In Neisseria gonorrhoeae, the best-characterized and most clinically important multidrug efflux system is the multiple transferrable resistance (MtrCDE) tripartite efflux pump, a member of the widely distributed resistance-nodulation-cell division (RND) superfamily in Gram-negative bacteria. N. gonorrhoeae MtrD contains multidrug binding sites and a proton relay network that generates the proton motive force (PMF) essential for drug expulsion from the bacterial cell. This multidrug efflux pump couples with the MtrC periplasmic membrane fusion protein and the MtrE outer membrane channel to actively extrude antimicrobials and mediate drug resistance. Based on the cryo-EM structures of MtrDCR103-CASP, MtrDCR103-Col, and MtrDCR103-LL, we observed that MtrDCR103 employs different binding modes to anchor linear and cyclic peptides.

To study MtrDCR103-Col interactions, we incubated 2 μM the MtrDCR103-nanodisc sample with 20 μM Col for 2 h to form the MtrDCR103-Col complex. We obtained a cryo-EM map of this complex at a 3.08-Å resolution. Similar to MtrDCR103-CASP, the structure of MtrDCR103-Col reveals an asymmetric trimer, with the three MtrDCR103 protomers exhibiting the access, binding, and extrusion conformational states. In the binding protomer of MtrDCR103, the cryo-EM map depicts an additional large density corresponding to the bound Col peptide. This bound Col molecule is found deep inside the distal drug binding site of the pump. The Col binding site overlaps that of CASP; however, it appears that MtrDCR103 utilizes a slightly different subset of residues to attach this peptide. Again, the nature of this protein-peptide interaction is mostly hydrophobic. Within 4.5 Å of this bound peptide, there are 26 residues, H46, S87, T128, S130, A132, S134, F136, I139, M141, Q172, R174, F176, S275, T277, A288, M290, P324, Y325, F568, I605, V607, F610, F612, S615, F623, and I625, that participate in facilitating Col binding. One notable difference is that some of the polar residues, such as S87, T128, S130, S134, Q172, and S615, do not interact with CASP. Presumably, these residues are more specific for Col recognition.

>MAKFFIDRPIFAWVISIFIIAAGIFGIKSLPVSQYPSVAAPTITLHAIYPGASAQVMEGSVLSVIERNMNGVEGLDYMSTSADSSGSGSVSLTFTPDTDENLAQVEVQNKLSEVLSTLPATVQQYGVTVSKARSNFLMIVMLSSDVQSTEEMNDYAQRNVVPELQRIEGVGQVRLFGAQRAMRIWVDPKKLQNYNLSFADVGSALSAQNIQISAGSIGSLPAVRGQTVTATVTAQGQLGTAEEFGNVILRANTDGSNIYLKDVAKVGLGMEDYSSSTRLNGVNTTGMAVMLSNSGNAMATAKAVKERLAVLEKYFPQGMSWKTPYDTSKFVEISIEKVIHTLIEAMVLVFVVMYLFLQNIRYTLIPTIVVPISLLGGFAFISYMGMSINVLTMFAMILVIGIVVDDAIVVVENVERIMAGEGLPPKEATKKAMGQISGAVIGITAVLISVFVPLAMFSGAAGNIYKQFALTMASSIAFSAFLALTLTPALCATMLKTIPKGHHEEKKGFFGWFNKKFDSWTHGYEGRVAKVLRKTFRMMVVYIGLAVVGVFLFMRLPTSFLPTEDQGFVMVSVQLPAGATKERTDATLAQVTQLAKSIPEIENIITVSGFSFSGSGQNMAMGFAILKDWNERTASGSDAVAVAGKLTGMMMGTLKDGFGIAVVPPPILELGNGSGLSINLQDRNNTGHTALLAKRNELIQKMRASGLFDPSTVRAGGLEDSPQLKIDINRAAAAAQGVSFADIRTALASALSSSYVSDFPNQGRLQRVMVQADGDARMQPADILNLTVPNSSGIAVPLSSIATVSWQMGTEQSVRFNGYPAMELSGSPATGVSTGQAMEAVQKMVDELGSGYSLEWGGQSREEAKGGSQTIALYALAAVAVFLVLAALYESWSIPLAVLLVMPLGLAGAAAGVTGRNLFEGLLGSVPSFANDIYFQVGFVTVMGLSAKNAILIIEFAKDLQAQGKSAVEAALEAARLRFRPIIMTSFAFILGVVPLYIAGGASSASQRAIGTTVFWGMLIGTLLSVFLVPLFYVVVRKFFKETAHE[3x];> XATAAALLAAT> GRPTKVFVPPFKT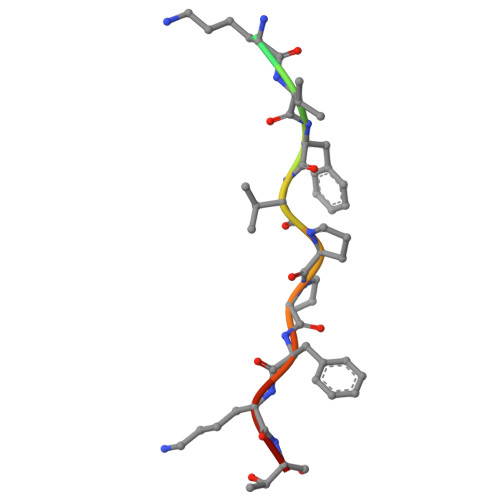K>[8x]EFRPEMLQGKKVIVTGASKGIGREMAYHLSKMGAHVVLTARSEEGLQKVVSRCLE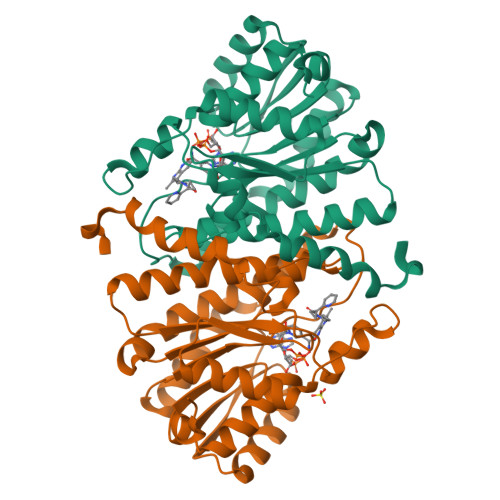LGAASAHYIAGTMEDMTFAEQFIVKAGKLMGGLDMLILNHITQTSLSLFHDDIHSVRRVMEVNFLSYVVMSTAALPMLKQSNGSIAVISSLAGKVTYPMVAPYSASKFALDGFFSTIRTELYITKVNVSITLCVLGLIDTETAMKAVSGIVNAQASPKEECALEIIKGTALRKSEVYYDKSPLTPILLGNPGRKIMEFFSLRYYNKDMF>[2x]HMVPMDKTLKEFGADVQWDDYAQLFTLIKDGAYVKVKPGAQTAIVNGQPLALQVPVVMKDNKAWVSDTFINDVFQSGLDQTFQVEKRPHPLNALTADEIKQAVEIVKASADFKPNTRFTEISLLPPDKEAVWAFALENKPVDQPRKADVIMLDGKHIIEAVVDLQNNKLLSWQPIKDAHGMVLLDDFASVQNIINNSEEFAAAVKKRGITDAKKVITTPLTVGYFDGKDGLKQDARLLKVISYLDVGDGNYWAHPIENLVAVVDLEQKKIVKIEEGPVVPVPMTARPFDGRDRVAPAVKPMQIIEPEGKNYTITGDMIHWRNWDFHLSMNSRVGPMISTVTYNDNGTKRKVMYEGSLGGMIVPYGDPDIGWYFKAYLESGDYGMGTLTSPIARGKDAPSNAVLLNETIADYTGVPMEIPRAIAVFERYAGPEYKHQEMGQPNVSTERRELVVRWISTVGNYDYIFDWIFHEN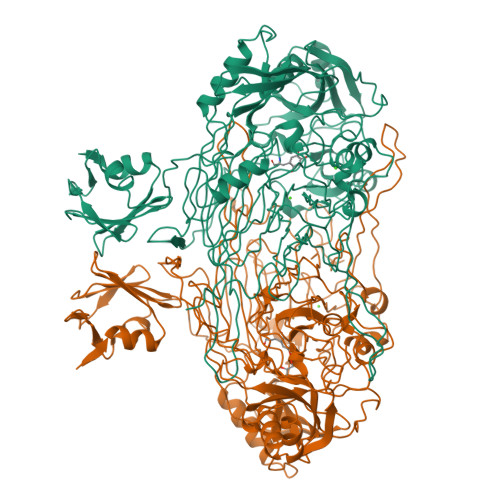GTIGIDAGATGIEAVKGVKAKTMHDETAKDDTRYGTLIDHNIVGTTHQHIYNFRLDLDVDGENNSLVAMDPVVKPNTAGGPRTSTMQVNQYNIGNEQDAAQKFDPGTIRLLSNPNKENRMGNPVSYQIIPYAGGTHPVAKGAQFAPDEWIYHRLSFMDKQLWVTRYHPGERFPEGKYPNRSTHDTGLGQYSKDNESLDNTDAVVWMTTGTTHVARAEEWPIMPTEWVHTLLKPWNFFDETPTLGALKKD>[8x]SGFVCNTCPEKWINFQRK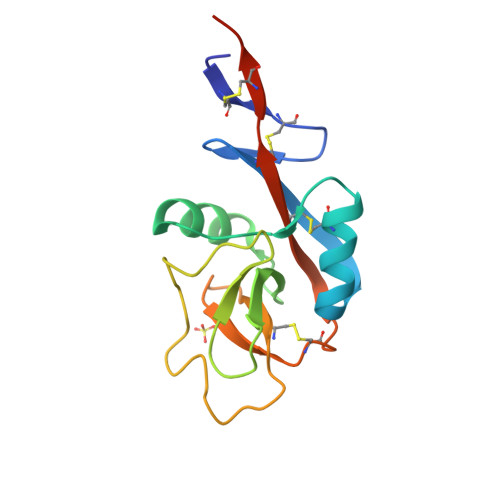CYYFGKGTKQWVHARYACDDMEGQLVSIHSPEEQDFLTKHASHTGSWIGLRNLDLKGEFIWVDGSHVDYSNWAPGEPTSRSQGEDCVMMRGSGRWNDAFCDRKLGAWVCDRLATCTPPASEGSAE>[2x]SNAMSTKTMKEKAVELLQKCEVVTLASVNKEGYPRPVPMSKIA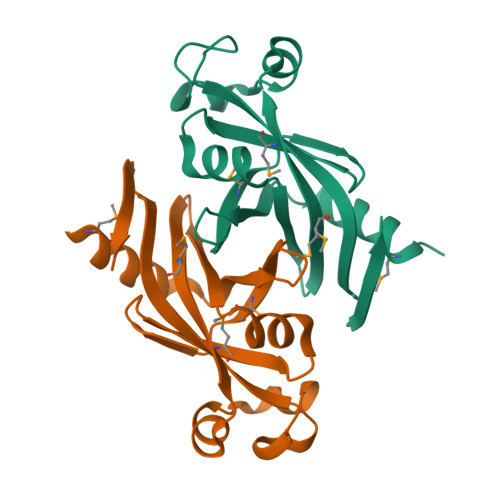AEGISTIWMSTGADSLKTIDFLSNPKAGLCFQEKGDSVALMGEVEVVTDEKLKQELWQDWFIEHFPGGPTDPGYVLLKFTANHATYWIEGTFIHKKLD7-(2-fluorobenzyl)quinolin-8-ol | 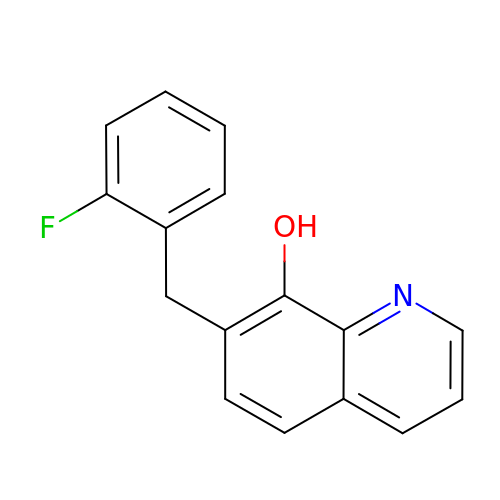C16 H12 F N O | HAPYRIFBEJEYED-UHFFFAOYSA-N> MCSTCANVLKYYNWDPHFRLVIDPNKFLSVGFCDNPLMCCYPELLPEFGTVWDCDQSPLQIYLESILGDDEWASTYEAIDPAVPPMHWDAAGKIFQPHPGVLMHHLIGEVAKAWDPNLPMFRLEADGDGSITAPEQGTPVGGVIAEPSAQMSAAADMATGKSVDSEWEAFFSFHTSVNWSTSETQGKILFKQSLGPLLNPYLEHLAKLYVAWSGSIDVRFSISGSGVFGGKLAAIVVPPGVDPVQSTSMLQYPHVLFDARQVEPVIFSIPDLRSTLYHLMSDTDTTSLVIMVYNDLINPYANDSNSSGCIVTVETKPGADFKFHLLKPPGSMLTHGSVPSDLIPKSSSLWIGNRHWTDITDFVIR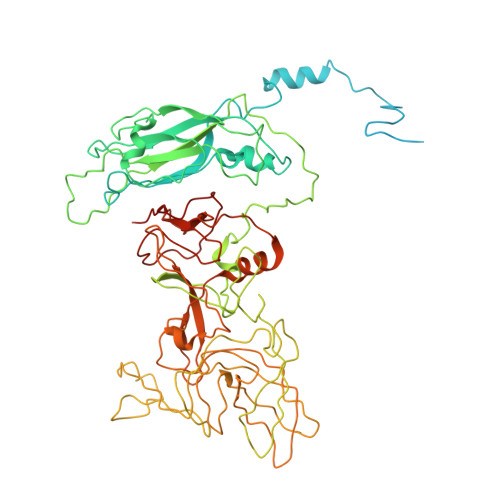PFVFQANRHFDFNQETAGWSTPRYRPITITISEKNGAKLGIGVATDYIVPGIPDGWPDTTIPEKLTPAGDYAITNKSGNDITTAAGYDGADVIVNNTNFKGMYICGSLQRAWGDKKISNTAFITTATKVDNAIEPSNVIDMTKIAVYQDTHVGKEVQTSDDTLSLLGYTGIGEQAIGSDRDRVVRISVLPETGARGGNHPIFYKNSIKLGYVIRSIDVFNSQILHTSRQLSLNHYLLPPDSFAVYRIIDSNGSWFDIGIDSDGFSFVGVSSIGKLEFPLTASYMGIQLAKIRLASNIRSSMTKL> GGSSRKSKAELQSEERKRIDELIESGKEEGMKIDLIDGKGRGVIATKQFSRGDFVVEYHGDLIE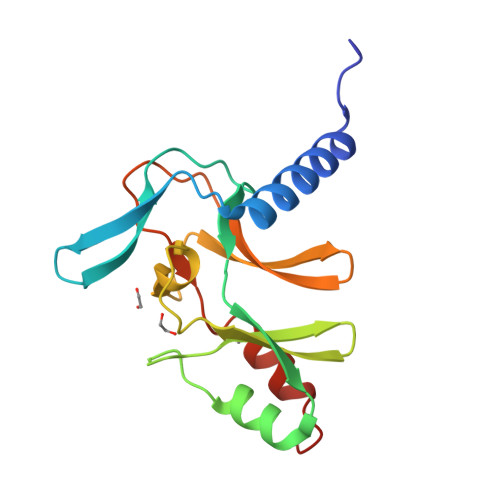ITDAAARAALYAQDPSTGCYMYYFQYLSKTYCVDATRETNRLGRLINHSKCGNCQTKLHDIDGVPHLILIASRDIAAGEELLYDYGDRSKASIEAHPWLKH> YQPNYFLSIPITNKKITAGIKVLQNSILRQDNRLTKAMVGDGSFHITLLVMQLLNEDEVNIGTDALLELKPFVEEILEGKHLTLPFHGIGTFQGQVGFVKLADGDHVSALLEIAE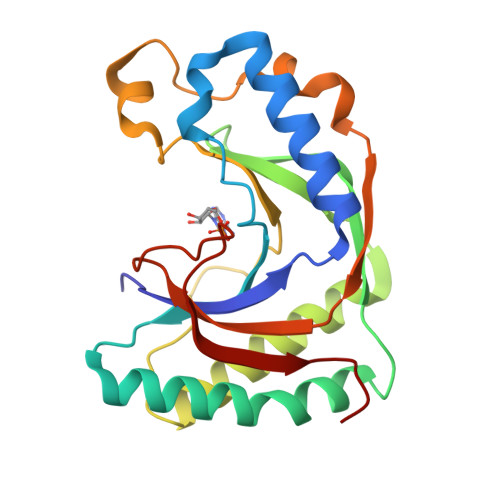TAKRTFQEKGILAGESRTFKPHLTFMKLSKAPMLWKKGVRKIEPGLYEQFIDHRFGEEILYQIDLCSMLKKKQSNGYYHCESSIVIGEKD> MEIVIRTGSGDVRGSKENGIAVFRGIPYAEPPVGAHRFTAPRPPRPWDGVRDATEFSATAPRPPYPEAIGALLIERFIPGDDYLTLNVWTPDPNAVGLPVMVWIHGGAFTNGSGSEPVYDGAAFARDGVVFVSFNYRLGIIGFADLPDAPSNRGLLDQIAALEWVRDNIARFGGDPGNVTVFGESAGAMSVCTLMATPRARGLFRRAILQSGAGNMAVAAEDATTIAAVIAHRLGVEPTAAALAHVPVAQLLDVQQQVAQEIQGAPD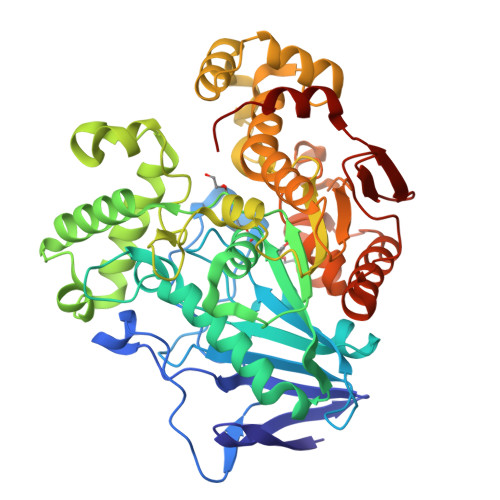PAVWGERIAGGSVLLPFAPVIDGELLSQRPAEAIAGGAGHDVDLLFGTTTDLYRLFLAPTGLLPFITSDYVTAHLAKSGLDADAAKAYTAEGRGEEPGDILASIITDQVFRIPALRIAESRVDAPARTFGYEFAWRTPQLDGILGACHAVELPFVFRTLDRAASLVGTNPPEELAETVHNAWVRFATSGDPGWPAWNPETRSVMRFDHPVSEMVTDPYPATRALWDGVPL>KLNSATSADEQPHIGNYRLLKTIGKGNFAKVKLARHILTGKEVAVKIIDKTQLNSSSLQKLFREVRIMKVLNHPNIVKLFEVIETEKTLYLVMEYASGGEVFDYLVAHGRMKEKEARAKFRQIVSAVQYCHQKFIVHRDLKAENLLLDADMNIKIADFGFSNEFTFGNKLDTFCGSPPYAAPELFQGKKYDGPEVDVWSLGVILYTLVSGSLPFDGQNLKELRERVLRGKYRIPFYMSTDCENLLKKFLILNPSKRGTLEQIMKDRWMNVGHEDDE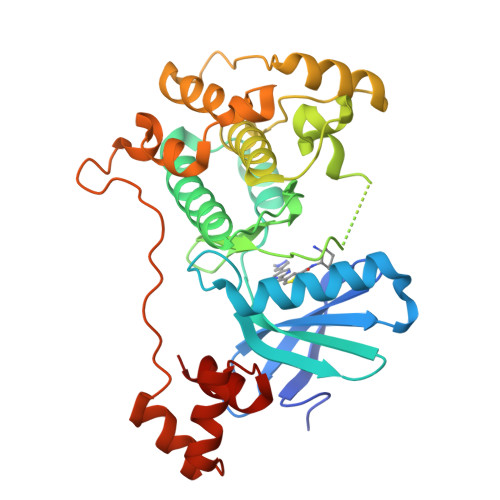LKPYVEPLPDYKDPRRTELMVSMGYTREEIQDSLVGQRYNEVMATYLLLGYK[2x]>MPDRTTDDFGPFTEQIRGTIDGMGTAEFDALPVGAIQVDGSGVIHRYNRTESRLSGRIPERVIGRNFFTEVAPCTNIPAFSGRFMDGVTSGTLDARFDFVFDFQMAPVRVQIRMQNAGVPDRYWIFVRK[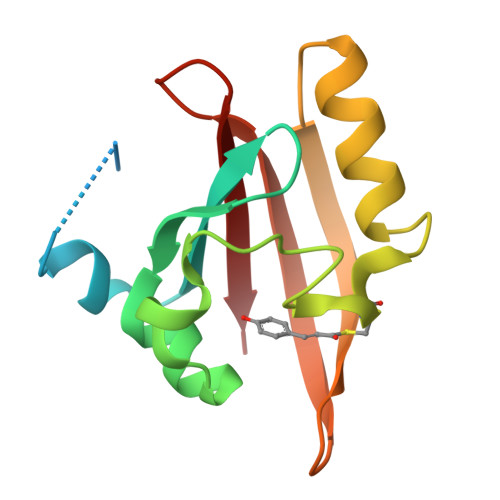3x]>[4x]MAHHHHHHMGAMKYVGALDQGTISTRFIIFDEKQCLVAQHQMPHRQLTPQAGWLEHDPMELYRASVACIVAAVEDLRRRVPSFEKLETIGIANQRETTVAWDRVTKETLYNAIVWSDLRSYEVTANVKKELGGGDDLFFAKMNGLRISTYFS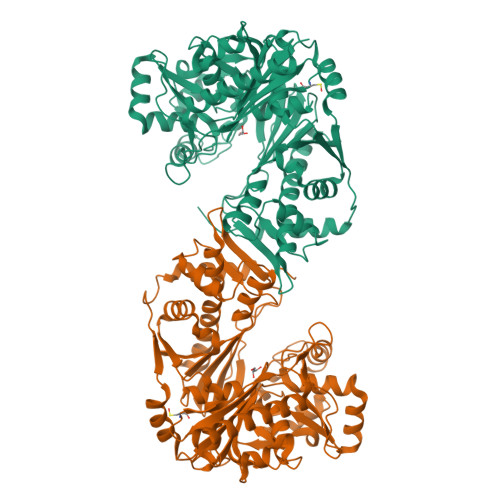AFKMRWMLENVPKVEEARKRGTLCFGTIDAWLLWKLSGGKVFVTDVTNASRTFLMDIRTCKWSPELCDKLGIPMACLPEIRSNSELFTYVLSDEGGLSTALRHPTPIMGSIADQQGALLGNMCFKEGESKNTYGTGCFLLMTVGERIRFSDHGLLSTVAYQLGNKSPFIYALEGSIAGAGATIEWLKNNMKLIDDVSDCEKFAQTVSDTQGVVFVPAFSGFLAPSWDPSARGSIFGMTLKTTRAHVLRAALLAIALQVVDVLEAMEKDAEVKVQFLRVDGGLTKNHLLMKMQSDLLGINLHRPTMAETTALGAALCAGLAAGVWKSLEEVKTISQQANVWRVIRPAASKDSQQMLRAQWKRAKQQAKWAKL> GPLGSKLTEMKCTNVVLLGLLSKMHVE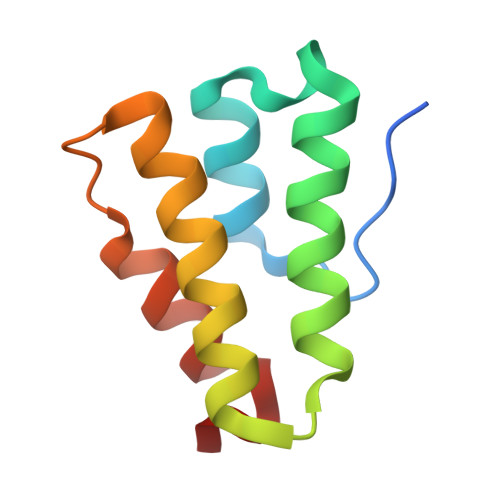SNSKEWNYCVGLHNEINLCDDPDAVLEKLLALIAFFLSKHNTCDLSDLIESYFENTTILQ>[2x]NNNGACUUAAGUCGG

Nonenzymatic template-directed RNA copying requires catalysis by divalent metal ions. The primer extension reaction involves the attack of the primer 3′-hydroxyl on the adjacent phosphate of a 5′-5′-imidazolium-bridged dinucleotide substrate. To explore the coordination of the catalytic metal ion with the imidazolium-bridged dinucleotide substrate, we examined catalysis by oxophilic and thiophilic metal ions with both diastereomers of phosphorothioate-modified substrates. High-resolution X-ray crystal structures of the products of primer extension with phosphorothioate substrates reveal the absolute stereochemistry of this interaction and indicate that catalysis by Mg2+ involves inner-sphere coordination with the nonbridging phosphate oxygen in the pro-SP position, while thiophilic cadmium ions interact with sulfur in the same position, as in one of the two phosphorothioate substrates.

We investigated the absolute stereochemistry of the product of Mg2+-catalyzed primer extension with phosphorothioate substrates by X-ray crystallography. We employed a partially self-complementary RNA 14-mer to establish a primer/template complex. Given that both the +1 and +2 positions on the template are locked 5-Me-C, only *psG was utilized as the substrate so that the Gps*psG bridged dimer was formed in situ either on the template or in solution followed by binding to the template. Although we used the two different diastereomeric *psG monomers, they ultimately result in the same (R, S)-Gps*psG substrate due to the inversion of chirality at one phosphorus center during the formation of the bridged dinucleotide. The resulting primer extension products were crystallized directly without further purification, and we were able to determine the structures of both product duplexes. Both products display stronger electron density at the upper position (upper sulfur) and weaker density at the lower position (lower oxygen). Therefore, both products have the same chirality (RP) on the +1 phosphorothioate, as expected. Furthermore, the RP chirality on the product (upper sulfur and lower oxygen) indicates that primer extension is possible only when the phosphate with lower oxygen and upper sulfur is bound at the +1 position. Given the oxophilic nature of Mg2+ ions, the lower oxygen content (pro-SP) plays a critical role in Mg2+ catalysis.>[2x]GVTKNNSCKKVGVEELINEKGCDLMIIRINRCRGHCFSFTFPNPLTKKYSVHAKCCRMVEWEMLETELKCSKGNRNLRIPSATQCECFDCLV;>GKECEFAMRLVPGFNPLRQVDA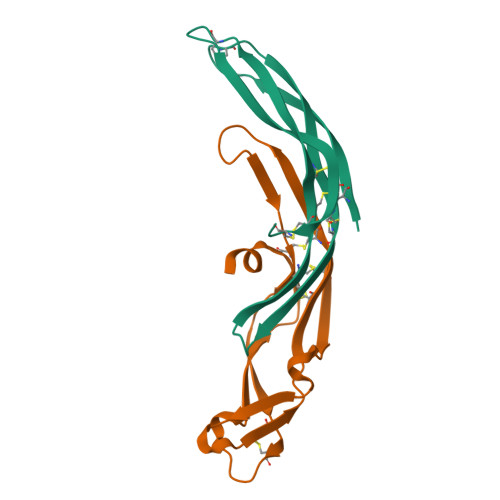NGKECRGNVELPFCKGYCKTSESGTHGFPPRVQNSKVCTLVTTSTRKVVLDDCDDGADESVKFVMVPHGTDCECSAVPLEQHHS[2x]> MSPNRFLLCVCILGLIAGGAAKVQYALTIPALLKSGETQRACVNLIGYHQPLALSVVLEHQRVNISIFSEKVQPPHYFKCNKFMVPTVITNAPDFVTLSVSGGGEDIKDRKAVVIAPLNTICLIQMDKPVYKPGCKVRFRLISLNTMLLPISEKYTAVYLEDPSGSRIAQWQNQESVGGVVQLEFPLISDAAPGSYTITAEGESCESARQGFTVDEYILPRFSVIVDPPNTISILDDILTLNVSAIYTYGQPVPGSVTIKCCREASSYYGRKGNCFKGNRGICTNITGELGPDGAFYGVVSLLPFQMGQSGFQMSLGVALTVTEEGT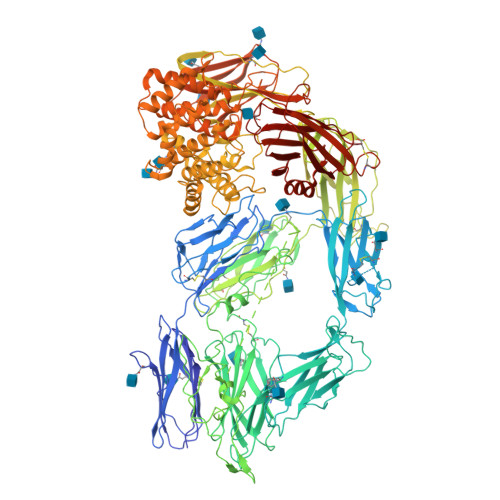GIQVTHQFFIMITSQLATLIFDYDALKEFYKRGIPYLVKVILTDANDNPMANEQVEVELAGKTIGAVLTDKEGRAEYAIDTSSFVQENFTVVVSYENPHQCYYTEWEGPDFPTAQHFVMRFYSETGSFLDIQGSSVELNCGQVHNISVRYILSLDGMGEGATTATFYYLAMSRAKIVQHGQRDVHLNQSKSGLFNIGLNVTSDLAPGAELIVYCILDLELIADTISLDIEKCFQNQVSLSFSDDLGPTASNVSLNLSAAPGSLCGVKVIDSSLLLINPYESLSASGVYYSIPYLSLFGYNYGGFNLEEPEPPCEDPNTVIFCKGRYYLPVSSSTEGDTYQNLRRVGLVLGTSSKIRKPVVCGMEAKFSVPRKSSGESDFGSSLSNGHVETLRKNFSETFLWRLVSVDSEGQNTITETVPDTITKWQGSMFCVSEKEGFGITKYSANFTSFLPFFVELSLPYSLTREEILVMKAFVSNYLEECIKIIVTLQPSADFEVIPQDVKQDQCICSGGRSSYSWNIIASSLGRISFIVSAETTHIGASCDGPSDQSQSTRKDTVIQTILVQPEGIRKEETSSNLVCVEDSNVEMPINLTLPENIVQGSASAFVTFVGDVLGLPLSNLQNLLQMPYGCGEQNLARMAPIPYVLEYLNNTNQLTDELLQTAVQFLNEGYYRQLRYKLPSGAYDAFWSSPSDGSSWLSAYTFKTFEKAKKYIYVDGKIQQQTLLYLQTSQKLDNGCFKAEGNLFMRQCGQERDLCFTAYLAIALLESNYSSGMTLLDDALGCLEAAMSSASTLYFKSYTVYVFTLVQNWEIRNTLLNELKSKVVSERGTLHWEREDKLGQEGIPLYYPNYSPAEVEITAYMLLSIAKGSDPTHDDLTYMAQISVWLIQQQNSYGGFRSTQDTVVALQALAFYAQLLFKSNAHHNVFLRSEYGDVGQLNLSEHNRLVVQRLQLPEVSGNYSISINGTGCCLVQSTIRYNIPVPKENSAFYVAADSVSKNCLNGVAYTITITVSVSYRGLRNETNMVIIDIQMLSGYQADYPSLRQLENSQQVSKTEEQDNHVFLYLNAVPLKTIQLSFKVLIGSRVLNVKSASVYVYDYYETGENGFASYSQPC>GHMAKGY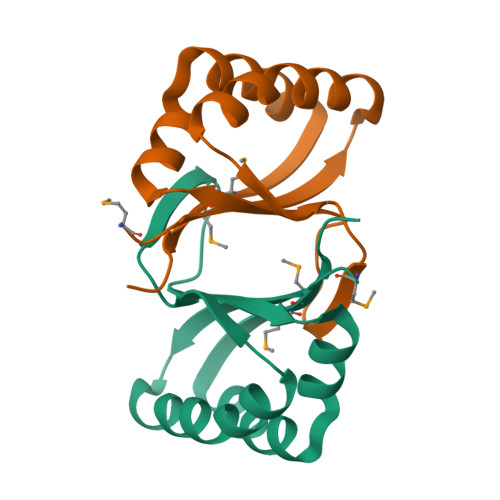WIAQVDVRDSERYKDYVSTAKPAFERFGANFLARGGSVTELEGTARARNVVIEFPSVQHAIDCYNSPEYQAAAKIRQEVADAEMMIVEGIGS[2x]> XV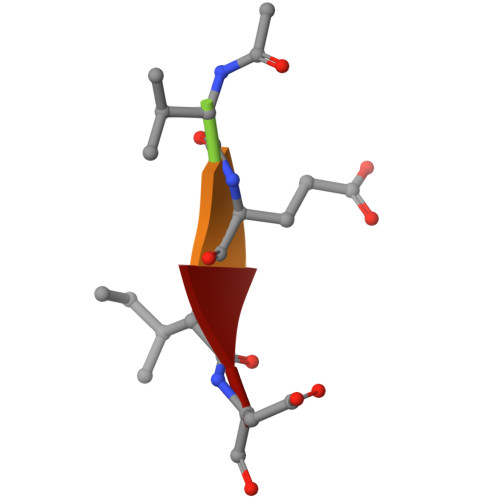EID>[4x]MDKFAEHEIPKAVIVAGNGESLSQIDYRLLPKNYDVFRCNQFYFEERYFLGNKIKAVFFTPGVFLEQYYTLYHLKRNNEYFVDNVILSSFNHPTVDLEKSQKIQALFID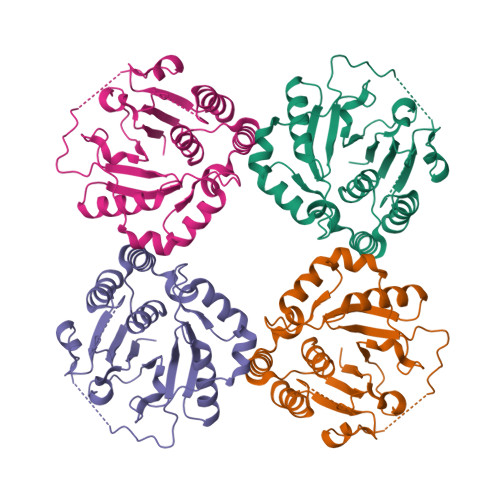VINGYEKHLSKLTAFDVYLRYKELYENQRITSGVYMCAVAIAMGYTDIYLTGIDFYQASEENYAFDNKKPNIIRLLPDFRKEKTLFSYHSKDIDLEALSFLQQHYHVNFYSISPMSPLSKHFPIPTVEDDCETTFVAPLKENYINDILLPPHFVYEKLGTIVSKKSRFHSNLIVRLIRDLLKLPSALKHYLKEK The first two steps in the pathway are catalyzed by the enzymes nicotine oxidoreductase (NicA2) and pseudooxynicotine amine oxidase (Pnao), which convert nicotine into pseudooxynicotine (Pon) and Pon into 3-succinoylsemialdehyde-pyridine, respectively. Both NicA2 and Pnao are members of the widespread flavin-dependent amine oxidase enzyme family. Enzymes of this family use a flavin adenine dinucleotide (FAD) prosthetic group to accept a hydride from their amine containing substrate, forming an oxidized product and reduced flavin hydroquinone (FADH2) in the reductive half reaction. However, our lab recently demonstrated that NicA2 is instead a dehydrogenase that uses a cytochrome c protein (called CycN) as a biological oxidant.

We were able to solve the structure of CycN at 1.9 Å, and the structure has a similar overall fold as bovine cytochrome c. We used rigid-body docking between CycN and Pnao and NicA2 and LHNO via the ZDOCK server to gain insight into how CycN may interact with these proteins. The ZDOCK server returns the top 10 docking poses as an output, and for Pnao, all 10 docking poses had CycN positioned in the same spot on the surface of Pnao. Docking CycN with the structure of NicA2 produced similar results, with eight of the top 10 docking poses having CycN positioned at the same relative location as that seen in the Pnao docking poses. Interestingly, this was not observed when we performed docking of CycN with LHNO; in that case, CycN was distributed across several positions on the surface of LHNO, with only one of the top 10 docking poses showing CycN at the common region observed with NicA2 and Pnao. This observation is consistent with the fact that LHNO reacts poorly with CycN and suggests that this common docking position observed with NicA2 and Pnao may correspond to the true CycN binding site for these enzymes. For example, Pnao contains Ser91, Phe98, Ser100, and Tyr422 on the surface of this potential binding site, and NicA2 contains identical residues at these positions. We previously observed that NicA2 and nicotine were unable to reduce bovine cytochrome c and noted that bovine cytochrome c has a much more positively charged surface than CycN on the heme-containing side of the protein. Yeast cytochrome c also has a similarly positively charged surface, and this difference in surface charge between CycN and bovine and yeast cytochrome c may, in part, be responsible for Pnao and NicA2’s specificity for CycN as a cytochrome c-based electron acceptor. Given how buried FAD is in the structure of Pnao, we suspect that CycN binds on the surface of Pnao, and the electrons on Pnao’s flavin are transferred to CycN over longer distances.

> DNCDPENGKKVYQICSVCHSNDTTGVHGAAAPNLHGLEGRKVGSVPGFKFSSALRDSGDTWTPQHLDKFLENPMAVYPLTRMAFSGLKNEKDRRDVLCFLSKSSN>[6x]MSLATPHINAQMGDFADVVLMPGDPLRAKYIAENFLDNAVQVCDVRNMFGYTGTYKGRRISVMGHGMGIPSCSIYVTELIKDYGVKKIIRVGSC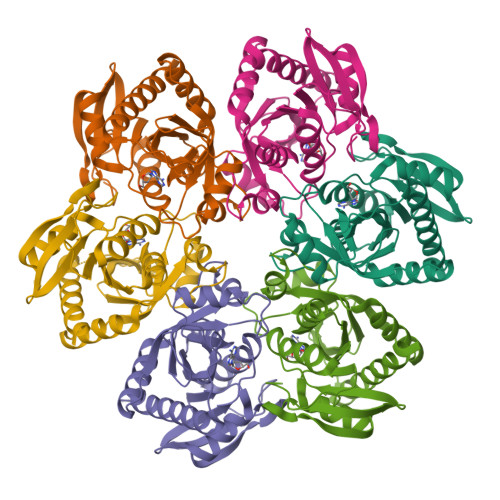GAVNEGIKVRDVVIGMGACTDSKVNRIRFKDHDFAAIADYKMVKAAEEAAKARGIDVKVGNLFSAELFYTPDPSMFDVMDKYGIVGVEMEAAGIYGVAAEYGAKALAICTVSDHIKTGEQTTSEERQNTFNEMIEIALDSVLIGDQAGYEGGSHHHHHH In this work, we exhaustively probe the ability of all 36 immobile HJ sequences to form DNA crystals in two different designed systems. Three separate self-assembling DNA crystal systems are described in this report: the “4 × 5” and “4 × 6” designs (collectively referred to as the 4 × N systems), and a third construct with a “scrambled” sequence variant of the 4 × 6 lattices. Self-assembly was mediated by three constituent oligonucleotides: (S1) containing four sequence repeats of either 5 or 6 bases; (S2) composed of 21 bases containing complementary regions to both (S1); and (S3) which forms the second junction crossover. The HJ serves as the fundamental component at the core of each unit, and the ultimate assembly of the full lattice is facilitated by the complementary 2-base sticky ends that tail each duplex.

The 4 × 5 system robustly crystallized with 75% of the junctions, and we obtained crystals in all but 9 of 36 sequences. Of the resulting structures, 18 exhibited P32 symmetry with average cell dimensions a = b = 68.85 Å c = 60.09 Å, with only nine retaining the original P3221 symmetry with average cell edges a = b = 68.17 Å c = 60.60 Å. Although the cell parameters between the two symmetries were virtually indistinguishable, the differences between the periodicity of the lattices is dramatic, with vastly different cavity sizes. Pos1 and 2 were readily observable in the electron density maps at either one or both of these conserved sites in a significant number of the structures, with no apparent respect to motif or symmetry. However, in the majority of the crystal structures reported here, the cacodylate anion indeed fits best into the electron density map of our X-ray structures, due to the presence of sodium cacodylate in the crystallization solution.

> GAGCAGACGTG;> ACTGCACTCA;> CAAGT;> TCTGAGTGCCGTCTGC>YKKAGLQRTLVLIKPDAFERSLVAEIMGRI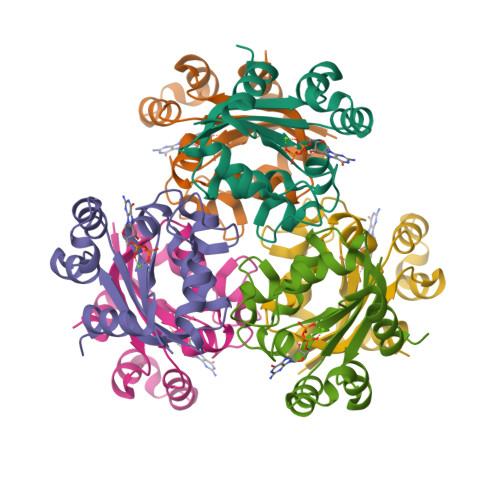EKKNFKIVSMKFWSKAPRNLIEQHYKEHSEQSYFNDNCDFMVSGPIISIVYEGTDAISKIRRLQGNTNPLASAPGTIRGDLANDIGENLIHASDSEDSAVDEISIWFPETKMETDN[2x]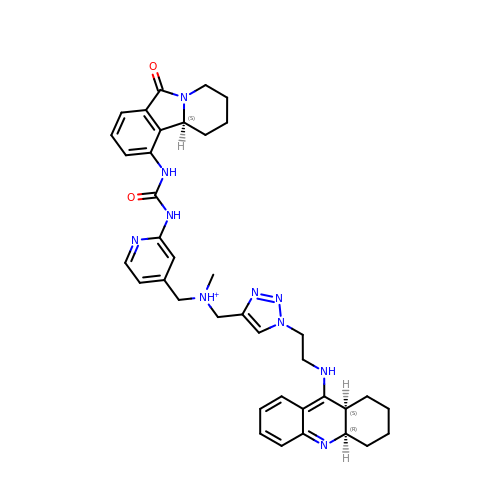[1-[2-(1,2,3,4,4~{a},9~{a}-hexahydroacridin-9-ylamino)ethyl]-1,2,3-triazol-4-yl]methyl-[[2-[[(10~{b}~{S})-6-oxidanylidene-2,3,4,10~{b}-tetrahydro-1~{H}-pyrido[2,1-a]isoindol-10-yl]carbamoylamino]pyridin-4-yl]methyl]-methyl-azanium | C38 H45 N10 O2 | FYSUEOXLAVKQLL-YVNFUZJASA-O>MNSGLSRLGIALLAAMFAPALLAADLEKLDVAALPGDRVELKLQFDEPVAAPRGYTIEQPARIALDLPGVQNKLGTKNRELSVGNTRSVTVVEAKDRTRLIINLTALSSYTTRVEGNNLFVVVGNSPHHHHHHHHAGASVASAAPVKASPAPASYAQPIKPKPYVPAGRAIRNIDFQRGEKGEGNVVIDLSDPTLSPDIQEQGGKIRLDFAKTQLPDALRVRLDVKDFATPVQFVNASAQSDRTSITIEPSGLYDYLVYQTDNRLTVSIKPMTTEDAERRKKDNFAYTGEKLSLNFQDIDVRSVLQLIADFTDLNLVASDTVQGN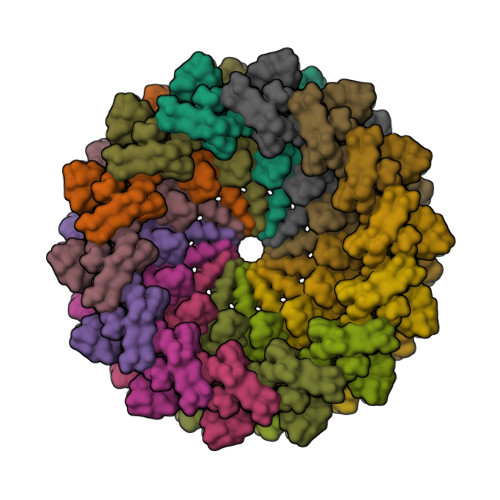ITLRLQNVPWDQALDLVLKTKGLDKRKLGNVLLVAPADEIAARERQELEAQKQIAELAPLRRELIQVNYAKAADIAKLFQSVTSDGGQEGKEGGRGSITVDDRTNSIIAYQPQERLDELRRIVSQLDIPVRQVMIEARIVEANVGYDKSLGVRWGGAYHKGNWSGYGKDGNIGIKDEDGMNCGPIAGSCTFPTTGTSKSPSPFVDLGAKDATSGIGIGFITDNIILDLQLSAMEKTGNGEIVSQPKVVTSDKETAKILKGSEVPYQEASSSGATSTSFKEAALSLEVTPQITPDNRIIVEVKVTKDAPDYQNMLNGVPPINKNEVNAKILVNDGETIVIGGVFSNEQSKSVEKVPFLGELPYLGRLFRRDTVTDRKNELLVFLTPRIMNNQAIAIGRGHHHHHHHH[14x]> NLYQFKNMIQCTVPSRSWADFADYGCYCGKGGSGTPVDDLDRCCQTHDNCYNEAENISGCRPKFKTYSYECTQGTLTCKG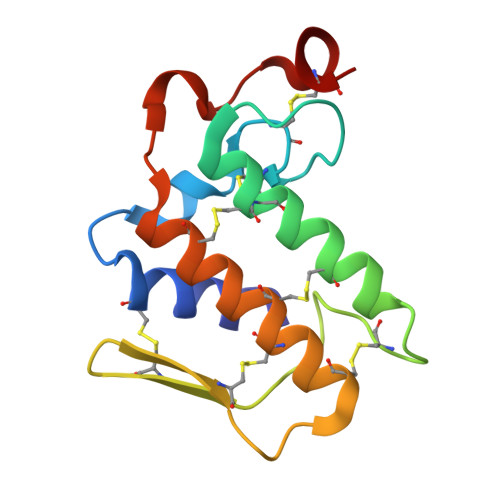DNNACAASVCDCDRLAAICFAGAPYNDANYNIDLKARCN> SGPINDTDANPRYKIPVE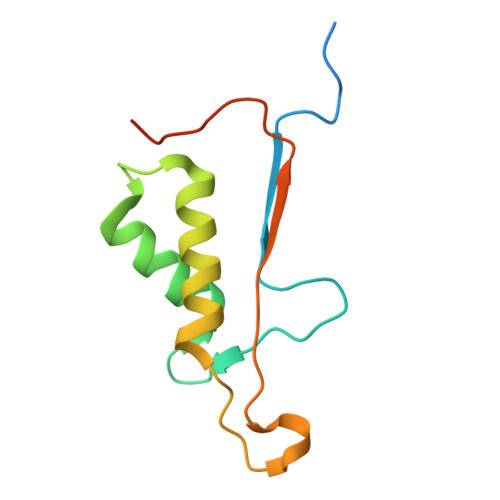ADFLFAYSTVPGYYSWRSPGRGSWFVQALCSILEEHGKDLEIMQILTRVNDRVARHFESQSDDPHFHEKKQIPCVVSMLTKELYFSQLEHHHHHH>PRERPHTSGHHGAGEARATAPSTVSPYGPEARAELSSRLTTLRNTLAPATNDPRYLQACGGEKLNRFRDIQCRRQTAVRADLNANYIQVGN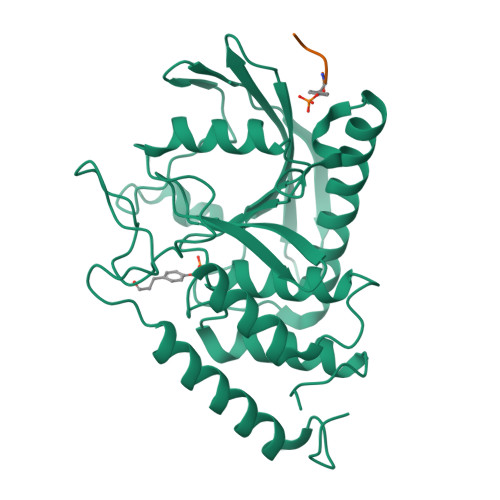TRTIACQYPLQSQLESHFRMLAENRTPVLAVLASSSEIANQRFGMPDYFRQSGTYGSITVESKMTQQVGLGDGIMADMYTLTIREAGQKTISVPVVHVGNWPDQTAVSSEVTKALASLVDQTAETKRNMYESKGSSAVADDSKLRPVIHSRAGVGRTAQLIGAMCMNDSRNSQLSVEDMVSQMRVQRNGIMVQKDEQLDVLIKLAEGQGRPLLNS[2x]>[2x]MHHHHHHQLHSVGKATQQMMQEPLTKERLISDWNSNVSVAVARTTAIAKSSDASLVQFLAADAAATTK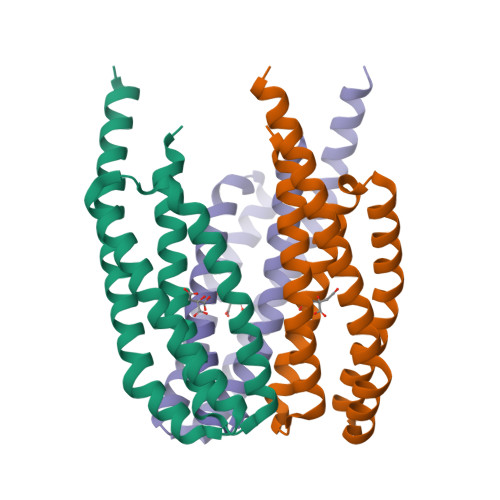STANVLKQIEPLITQPAEREILDKIMQVRKTYIASRDKVSQLKADGMAEEAESTLINSYVPAAQGYLKLLGELLNLQRASLDAKAAEVEQIESSSRT>MRGSHHHHHHGSPGLQEFMAATGANAEKAESHNDCPVRLLNPNIAKMKEDILYHFNLTTSRHNFPALFGDVKFVCVGGSPSRMKAFIRCVGAELGLDCPGRDYPNICAGTDRYAMYKVGPVLSVSHGMGIPSISIMLHELIKLLYYARCSNVTIIRIGTSGGIGLEPGTVVITEQAVDTCFKAEFEQIVLGKRVIRKTDLNKKLVQELLLCSAELSEFTTVVGNTMCTLDFYEGQGRLDGALCSYTEKDKQAYLEAAYAAGVRNIEMESSVFAAMCSACGLQAAVVCVT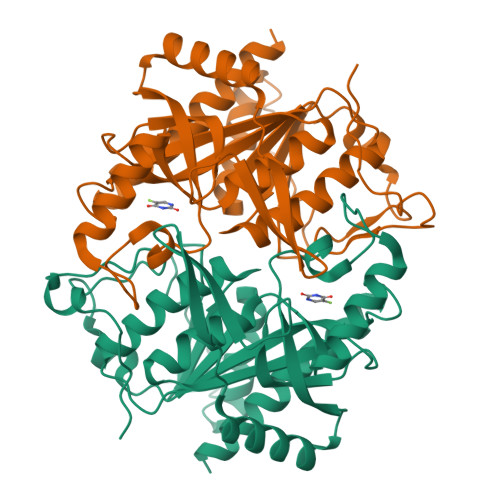LLNRLEGDQISSPRNVLSEYQQRPQRLVSYFIKKKLSKA[4x]> KKKGSVVIVGRINLSGDTAYAQQTRGEEGCQETSQTGRDKNQVEGEVQIVSTATQTFLATSINGVLWTVYHGAGTRTIASPKGPVTQMY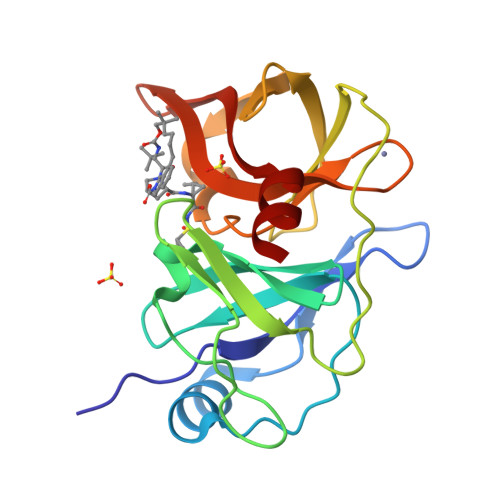TNVDKDLVGWQAPQGSRSLTPCTCGSSDLYLVTRHADVIPVRRRGDSTGSLLSPRPLSYLKGSSGGPLLCPAGHAVGIFRAAVSTRGVAKAVQFIPVESLETTM> QNTVNFTYPDFWSYSLKNGTEITFLGDATRIPGALQLTKTDANGNPVRSSAGQASYSEPVFLWDSTGKAASFYTSFTFLLKNYGAPTADGLAFFLAPVDSSVKDYGGFLGLFRHETAADPSKNQVVAVEFDTWINKDWNDPPYPHIGIDVNSIVSVATT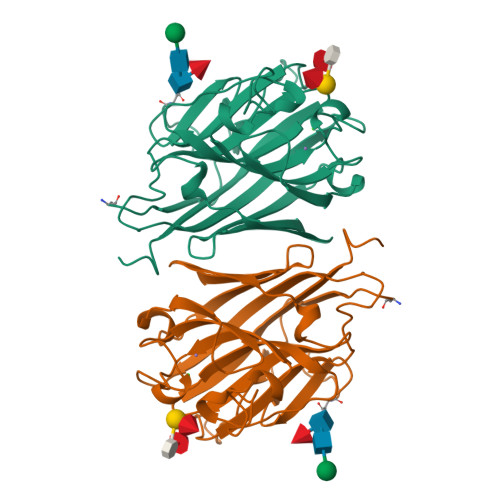RWENDDAYGSSIATAHITYDARSKILTVLLSYEHGRDYILSHVVDLAKVLPQKVRIGFSAGVGYDEVTYILSWHFFSTLDGTNK> MKPERKRVSKLMAYILRHSP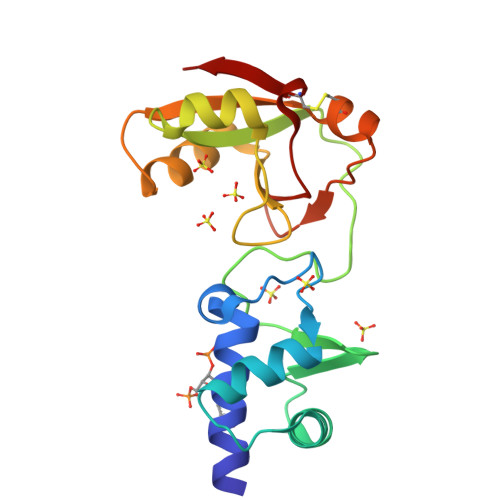EEFGLRPDVEGFVSLNELVNALKTVYPEVTEEFVREIVENDPKGRYEIRGDRIRARYGHSFPVSLDHEEDTESRFLYHGTPRRNLPSILKEGLKPMKRQYVHVSTDKIEALETGRRHGREVVLLVIDAECLRKRGFKIYKAGKNVRIVERVPPDCITLAV>MRTSKKEMILRTAIDYIGEYSLETLSYDSLAEATGLSKSGLIYHFPSRHALLLGMHELLADDWDKELRDITRDPEDPLERLRAVVVTLAENVSRPELLLLIDAPSHPDFLNAWRTVNHQWIPDTDDLENDAHKRAVYLVQLA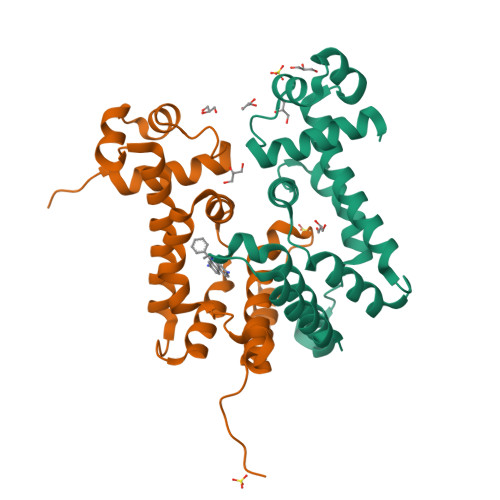ADGLFVHDYIHDDVLSKSKRQAMLETILELIPSELHHHHHH[2x]> SLGNKLSITDVKAIQGKKVLVRVDFNVPIENGVIKDTNRITATLPTIHHLKKEGAAKIILISHCGRPDGT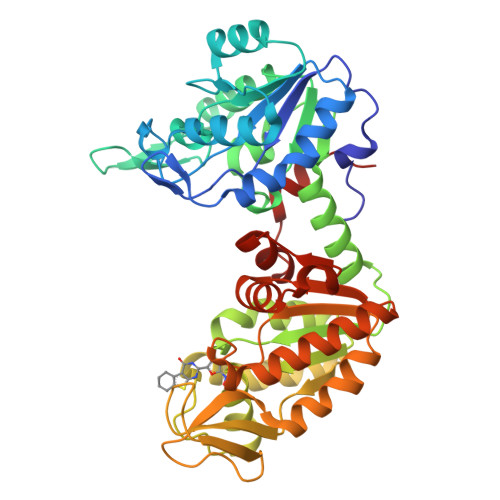KNLKYTLKPVAETLGTLLGEEVLFLSDCVGEEVAAQINQAKDNSVILLENLRFHVEEEGKGVDAAGNKIKASKEDMEKFQNELTKLGDVFINDAFGTAHRAHSSMVGIKMNVKASGFLMKKELEYFSKALENPQRPLLAILGGAKVSDKIQLIKNLLDKVDKMIIGGGMAYTFKYVLNNMKIGDSLFDEAGSKIVNEIMEKAKAKNVEIYLPVDFKVADKFDNNANTKVVTDEEGIEDKWMGLDAGPKSIENYKDVILSSKTIIWNGPQGVFEMPNFAKGSIECLNLVIEATKKGAISIVGGGDTASLVEQQQKKNEISHVSTGGGASLELLEGKELPGVVALSSK> MAQDALSDGFVRLCIDPSLNFFGEGCKILVEGQMTDDGSATPDAVTCVTSELDIIERFGQGSVLTESLRKVFCTCKSGVSVYALPREDAAAGVKAVYTLTIAGPATTDGRVQLYMGEAEYAVDIGVDAGDTATDIAAAIVAAISPDFPYAATAAAGVITLTARNAGTIGNHLSVIYTNLGSCTSVTPEGVTVTFAQTTAGSVNPTPNDYATVVNECCFAVYVLSSDDTDWQENLRDWIRSAWDCSKPQCFGHGYVFNKGTLGQVLADGDNSAELSRLALPTTYPVLPYLTNAAYGALSACSTCNNPELNIQGQTFGLLSCINMPESCTPGWTFGEVTQLQANGFVVSGPSTTSGQGNYTSPYIYNDVTNYLRDEKNRPNATFRDASSRRLAAATGVALAEFLQQFNGLAVFTKNTNIRTGIIGTNPRLMLGKIRKWAQDNVGTLFSEFDNINEDIQLLTDFEVQPKCVGQPGIFHLNMRYRPPVR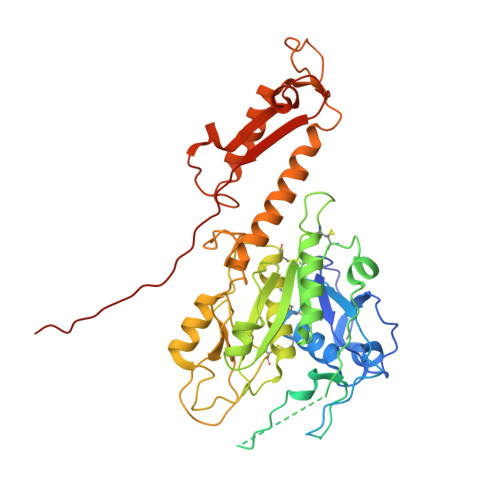GARINVNMAPALFDNCDR> SNAEKETGSKELAKVDGNVTIKDLSFAFGEHKVLSGVSVDIKAGQTVAFVGKS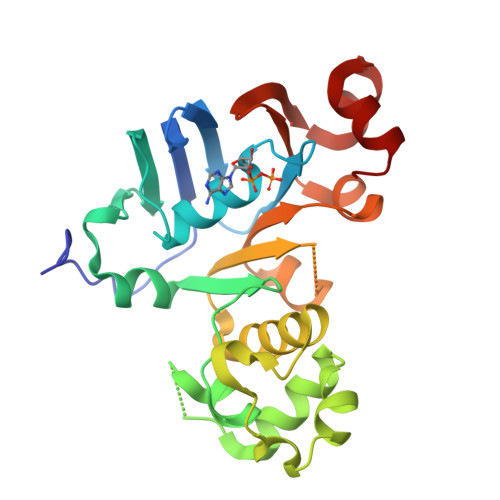GSGKTTLTSIISRFYTQHEGEILLDGVDTRELTLENLRSHLSIVSQNVHLFDDTVYNNIAFGLSREVSEEEVIDALKRANAYEFVQELSDGINTNIGNNGSKLSGGQRQRISIARALLKNAPVLIFDEATSALDNESERVVQQALESLTKSCTTIVIAHRLSTVENADKIVVMDGGRVVESGKHQELLEQGGLYTRLYQSGLQ Btk is critical for the generation of calcium flux in response to receptor activation, because it activates phospholipase C-γ2 (PLC-γ2), which produces the second messengers diaceylglycerol (DAG) and inositol (1,4,5)-trisphosphate (IP3). Btk dysfunction is the cause of X-linked agammaglobulinemia, a severe disease of primary immunodeficiency. The Tec family kinases have a lipid-interaction module attached to the N terminus of a Src-like module (i.e., concatenation of an SH3 domain, an SH2 domain and a tyrosine kinase domain). The lipid-interaction module of the Tec kinases is an extended plekstrin homology (PH) domain fused to a Tec homology (TH) domain.

We replaced six residues in the activation loop of Btk with the corresponding ones in Itk, shown previously to stabilize the activation loop of the Btk kinase domain. The overall conformation of the kinase domain, as well as the specific conformation of the activation loop, is very similar in the two structures we have determined. We also determined the structure of the isolated Btk kinase domain with the six mutations described above and found by comparing it to wild-type Btk that the mutations do not introduce major perturbations in the structure. The kinase domain of Btk has low catalytic activity and autophosphorylates very slowly, like the c-Abl kinase domain and unlike those of the Src family. For example, there is no detectable change over 90 min in the level of phosphorylation of the Btk kinase domain at 4 μM concentration. IP6 has no effect on activation of the isolated kinase domain of Btk, suggesting that it is not a direct allosteric activator of the enzyme.

>[4x]AWEIDPKDLTFLKELGTGQFGVVKYGKWRGQYDVAIKMIKEGSMSEDEFIEEAKVMMNLSHEKLVQLYGVCTKQRPIFIITEYMANGCLLNYLREMRHRFQTQQLLEMCKDVCEAMEYLESKQFLHRDLAARNCLVNDQGVVKVSDFGMTRFVLDDEYTSSTGTKFPVKWASPEVLMYSKFSSKSDIWAFGVLMWEIYSLGKMPYERFTNSETAEHIAQGLRLPRPHLASERVYAIMYSCWHEKADERPTFKILLSNILDVMDEES(2R)-14-fluoro-2-methyl-6,9,10,19-tetrazapentacyclo[14.2.1.02,6.08,18.012,17]nonadeca-1(18),8,12(17),13,15-pentaen-11-one | C16 H15 F N4 O | 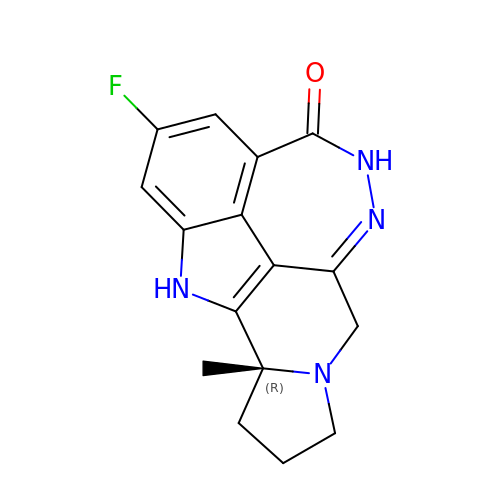DENYZIUJOTUUNY-MRXNPFEDSA-N> MEAGITGTWYNQ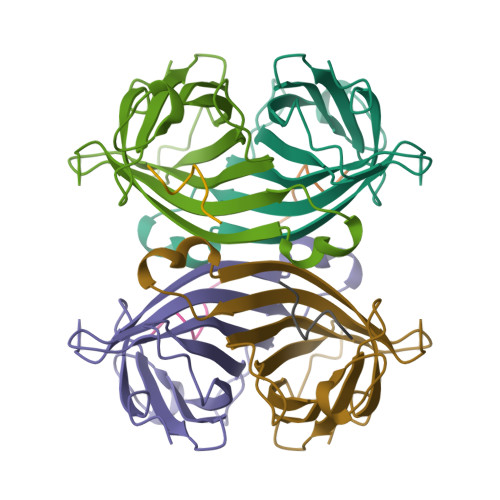LGSTFIVTAGADGALTGTYESAVGNAESRYVLTGRYDSAPATDGSGTALGWTVAWKNNYRNAHSATTWSGQYVGGAEARINTQWLLTSGTTEANAWKSTLVGHDTFTKVKPSAAS;> SNWSHPQFEK> MSNAALATAPHALELDVHPVAGRIGAEIRGVKLSPDLDAATVEAIQAALVRHKVIFFRGQTH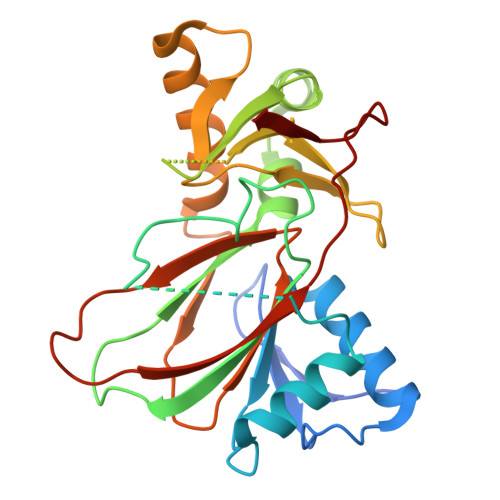LDDQSQEGFAKLLGEPVAHPTVPVVDGTRYLLQLDGAQGQRANSWHTDVTFVEAYPKASILRSVVAPASGGDTVWANTAAAYQELPEPLRELADKLWAVHSNEYDYASLKPDIDPAKLERHRKVFTSTVYETEHPVVRVHPISGERALQLGHFVKRIKGYSLADSQHLFAVLQGHVTRLENTVRWRWEAGDVAIWDNRATQHYAVDDYGTQPRIVRRVTLAGEVPVGVDGYLSRTTRKG(2Z)-3-(6-bromo-1H-indol-3-yl)-2-sulfanylprop-2-enoic 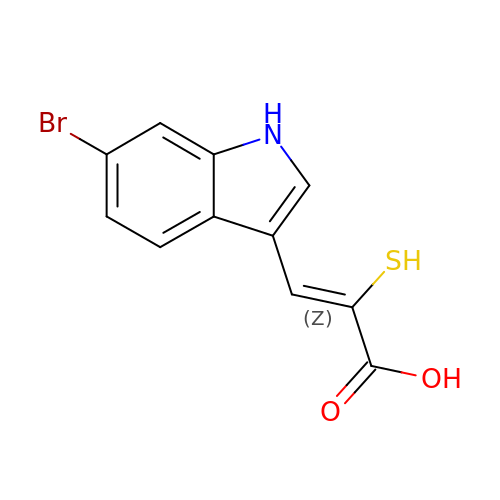acid | C11 H8 Br N O2 S | BTHAZQKLFQMXOX-KMKOMSMNSA-N>MNMPMTERIRAGKLFTDMCEGLPEKRLRGKTLMYEFNHSHPSEVEKRESLIKEMFATVGENAWVEPPVYFSYGSNIHIGRNFYANFNLTIVDDYTVTIGDNVLIAPNVTLSVTGHPVHHELRKNGEMYSFPI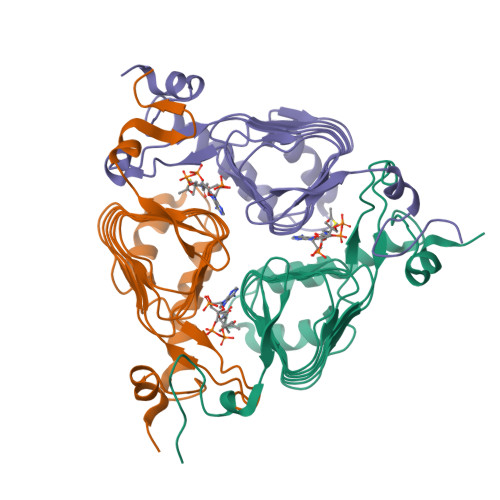TIGNNVWIGSHVVINPGVTIGDNSVIGAGSIVTKDIPPNVVAAGVPCRVIREINDRDKHYYFKDYKVESSV[3x]> MEL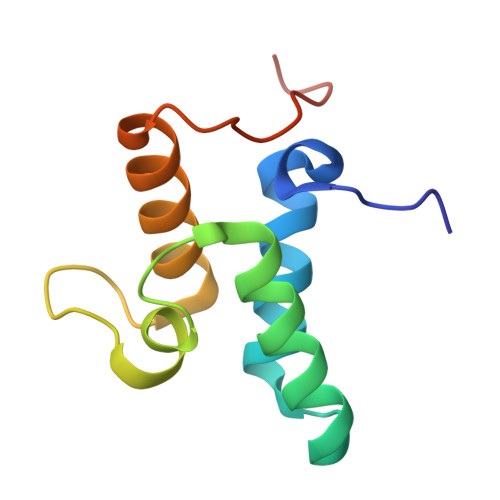KHSISDYTEAEFLEFVKKIEDANSSEDEQQKLVEEFIRLTEHPSGSDLIYYPRDDREDSPEGIVKEIKEWRAANGKSGFKQGLEHHHHHH>[2x]HHHHHHFNLPPGNYKKPKLLYCSN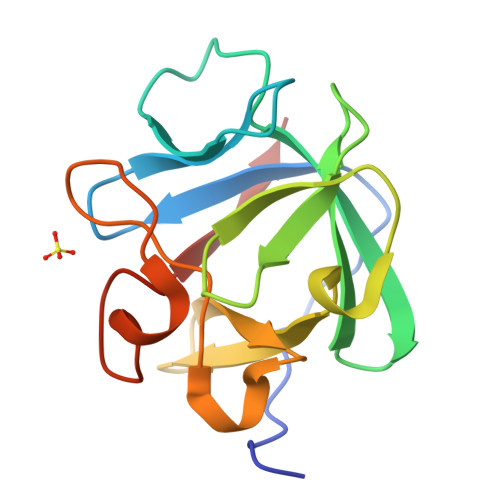GGHFLRILPDGTVDGTRDRSDQHIQWQLSAESVGEVYIKSTETGQYLAMDTDGLLYGSQTPNEECLFLERLEENHYNTYISKKHAEKNWFVGLKKNGSCKRGPRTHYGQKAILFLPLPVSSD> GPMQPRLKVGAIPDQNPERLNRLYGQLADELSDRLNVKVRYVPVSNYPAAVSAFRTGGLDLVWFGGLTGVQARLQTPGAQVLAQRDIDARFRSVFIANTSSGLQPISSINGLTSLRGKRFSFGSESSTSGRLMPQHFLAKAGVTPSQFSGGRAGFSGSHDATIAVVQSGAYEAGALNEQVWTSAVNDGRVNTEKVSVIWRTPEYVDYHWVVRPKLDQRFGKGFT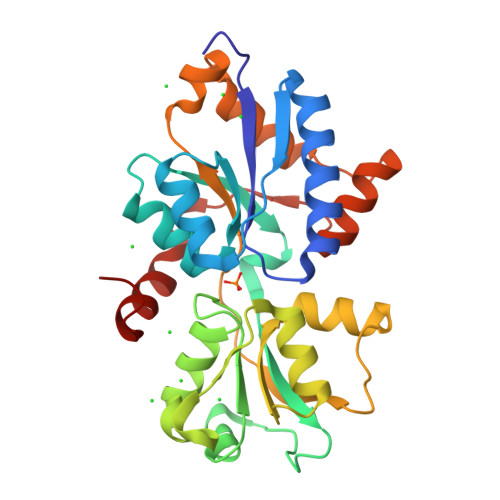TRLQKAILGLEPTTPRQVTILELFAAKRFIPVEASQYKPIEKVGRELGKIR>MKTHILLARVLACAALVLVTPGYSSEKIPVTGSGFVAKDDSLRTFFDAMALQLKEPVIVSKMAARKKITGNFEFHDPNALLEKLSLQLGLIWYFDGQAIYIYDA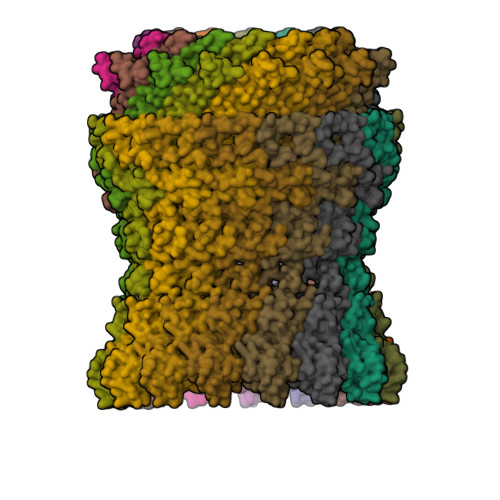SEMRNAVVSLRNVSLNEFNNFLKRSGLYNKNYPLRGDNRKGTFYVSGPPVYVDMVVNAATMMDKQNDGIELGRQKIGVMRLNNTFVGDRTYNLRDQKMVIPGIATAIERLLQGEEQPLGNIVSSEPPAMPAFSANGEKGKAANYAGGMSLQEALKQNAAAGNIKIVAYPDTNSLLVKGTAEQVHFIEMLVKALDVAKRHVELSLWIVDLNKSDLERLGTSWSGSITIGDKLGVSLNQSSISTLDGSRFIAAVNALEEKKQATVVSRPVLLTQENVPAIFDNNRTFYTKLIGERNVALEHVTYGTMIRVLPRFSADGQIEMSLDIEDGNDKTPQSDTTTSVDALPEVGRTLISTIARVPHGKSLLVGGYTRDANTDTVQSIPFLGKLPLIGSLFRYSSKNKSNVVRVFMIEPKEIVDPLTPDASESVNNILKQSGAWSGDDKLQKWVRVYLDRGQEAIK[15x]> GPHMATGQDRVVALVDMDCFFVQVEQRQNPHLRNKPCAVVQYKSWKGGGIIAVSYEARAFGVTRSMWADDAKKLCPDLLLAQVRESRGKANLTKYREASVEVMEIMSRFAVIERASIDEAYVDLTSAVQERLQKLQGQPISADLLPSTYIEGLPQGPTTAEETVQKEGMRKQGLFQWLDSLQIDNLTSPDLQLTVGAVIVEEMRAAIERETGFQCSAGISHNKVLAKLACGLNKPNRQTLVSHGSVPQLFSQMPIRKIRSLGGKLGASVIEILGIEYMGELTQFTESQLQSHFGEKNGSWLYAMCRGIEHDPVKPRQLPKTIGCSKNFPGKTALATREQVQWWLLQLAQELEERLTKDRNDNDRVATQLVVSIRVQGDKRLSSLRRCCALTRYDAHKMSHDAFTVIKNCNTSGIQTEWSPPLTMLFLCATKFSAS

DNA polymerase η (Pol η) is a Y-family polymerase involved in DNA translesion synthesis against UV-induced lesions. Despite their various biological roles and subunit compositions, all DNA polymerases contain similar active sites and catalyze the metal-ion dependent nucleotidyl transfer reaction via similar kinetic pathways. The A-site metal ion (Me2+A) bridges the primer 3′-OH and the substrate α-phosphate to promote deprotonation and nucleophilic attack, while the B-site metal ion (Me2+B) stabilizes the triphosphate motif of the incoming deoxynucleotide triphosphate (dNTP). Using X-ray time-resolved crystallography, we visualize the complete DNA misincorporation process catalyzed by DNA polymerase η.

To start the reaction, we equilibrated Pol η crystals at pH 7.0 and then soaked the crystals in reaction buffer containing Mg2+ or Mn2+. Within the active site, the incorrect dGTP was assigned with 80% occupancy according to its density. In the ground state, t = 0 s, the Me2+A site was occupied at 30% by a monovalent K1+, and the Me2+B site was occupied at 80% by a divalent Ca2+. In the up conformation, the primer 3′-OH was located 3.7 Å above the substrate α-phosphate while the sugar moiety interacted with R61. In the down conformation, the 3′-OH existed 3.6 Å away from the K1+ and 3.3 Å away from S113. Assigning 15% of the 3′-OH in the down conformation eliminated any significant Fo-Fc peaks around the primer terminus. Regarding base-pair geometry of our mismatch structure, the incorrect substrate dGTP and template dT formed a wobble base-pair, in which the base of the incoming dGTP shifted 1.6 Å towards the minor groove while the template dT shifted 0.9 Å towards the major groove, compared to the ground state structure with the correct substrate dATP. Hydrogen bonds between dGTP and the protein sidechains Q38 and R61 possibly stabilized the wobble base-pair. Furthermore, due to the wobble base geometry, there was a reduction in pi-stacking interactions between the incoming dGTP and primer aromatic base. At this point, the majority of the primer 3′-OH exists in the up conformation not aligned with the α-phosphate of dGTP, and most of the R61 sidechain is interacting with the wobble base-pair.>MSDPTHLISKRAAGRTSVHFTNAPSDKPPANFKPHEKPLALSYGMPNHGFFPIDSIDVNLVDYPFQKITTPSTTSSTAEEEPPSSSLNGSENGHQTKTPPSSIHTPQSTVHISRHTTDPKLIDLARGLQYAAVEGHAPLLQFARDFIIRTHKPNYDDWNVFITTGASDGLNKAADVFLDDGDVILVEEFTFSPFLRFSDNAGAKAVPVKINFDNDSDGIDLTQFVDLLENWEKHYPNLPKPKALYTIATGQNPTGFTQSL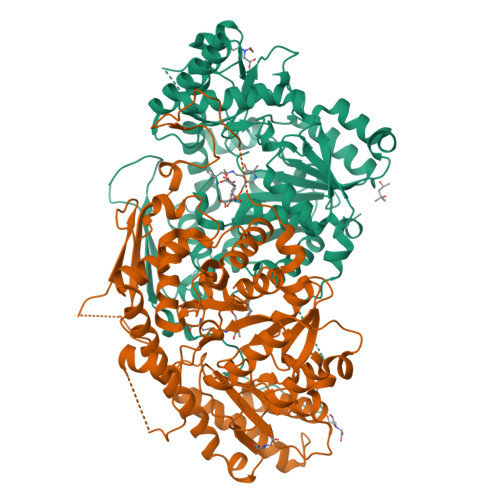EFRKKIYDLAVKYDFAIIEDDPYGYLTLPKYEKPNIGGSGSGNNELKNDLEIDDYLKNHLTPSYLELDTTGRVLRVETFSKLFAPGLRLGFIVGHKEVIDAVKNYSDVVNRGASGLTQTIVNNVIQENFKGVDGWLEWILKMRLNYSYRKDLLLYSIFESQAYKKGYVDVIDPKAGMFVTFKINLPKDVDVLQKMKLLLWKLISYGILVVPGYNMTVDLEFSKDRSNFFRLCYALANNDEEILESGKRLTDAVYEFFSNGLEFH[2x]>[2x]SNAIRDISSIELIKEMRFGWNLGNTLDAECTSWMDYEKNPIGSETCWGNVKTNEDIFKTLMDNQFNVFRIPTTWTGHIGEAPEYKINEQWMKRVHEIVDYPYKNGAFVILNIHHETWNHAFAETVDEA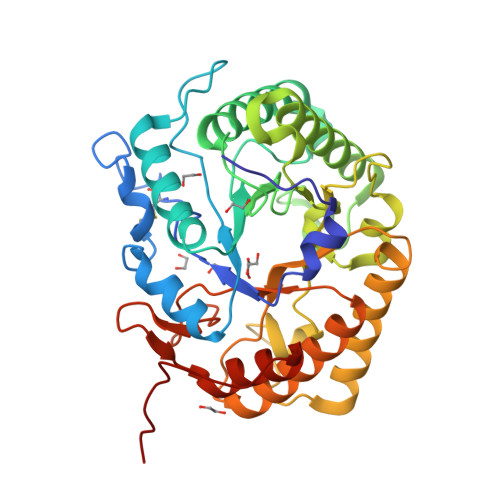KVELAQVWKQIAEEFKGYGERLIFEGQNEPRKNGTPVEWNGGDKEGWDVVNAMNAVFLETVRSSGGNNAKRHLMIPPYAAACNENSFKNFDFPEDDDKVIASVHAYSPYNFALNNGEGAVDKFDASGKNELDWNINLMKKRFVDQGIPMILGEYGAMNRDNEEERAAWAEYYMEKITALGVPQVWWDNGVFEGEGERFGLIDRKNLKIVYPSIVAALQKGRGLEVNVLHAIETEPEE>[6x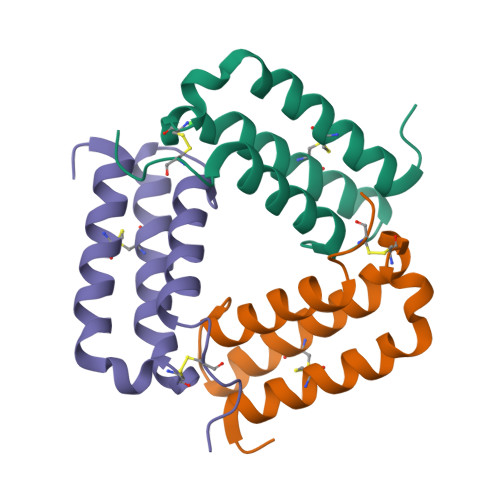]SMTGTPGSEGGTVKNYETAVQFCWNHYKDQMDPIEKDWCDWAMISRPYSTLRDCLEHFAELFDLGFPNPLAERIIFETHQIHFANCSLVQPTFS>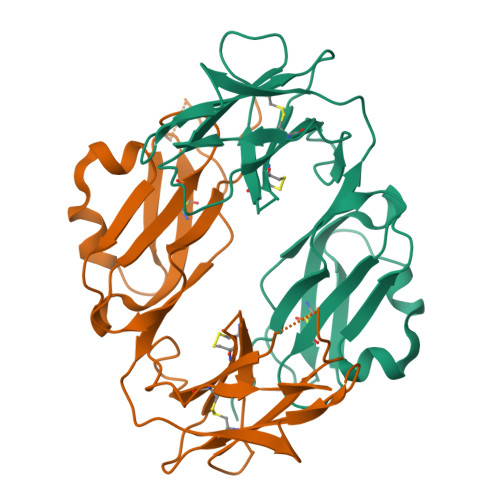[2x]GHLPKPTLWAEPGSVITQGSPVTLRCQGGQETQEYRLYREKKTALWITRIPQELVKKGQFPIPSITWEHAGRYRCYYGSDTAGRSESSDPLELVVTGAYIKPTLSAQPSPVVNSGGNVILQCDSQVAFDGFSLCKEGEDEHPQCLNSQPHARGSSRAIFSVGPVSPSRRWWYRCYAYDSNSPYEWSLPSDLLELLVL> FSNKRVLVEKEGEAGIAVMKFKNPPVNSLSLEFLTEFVISLEKLENDKSIRGVILTSERPGIFSAGL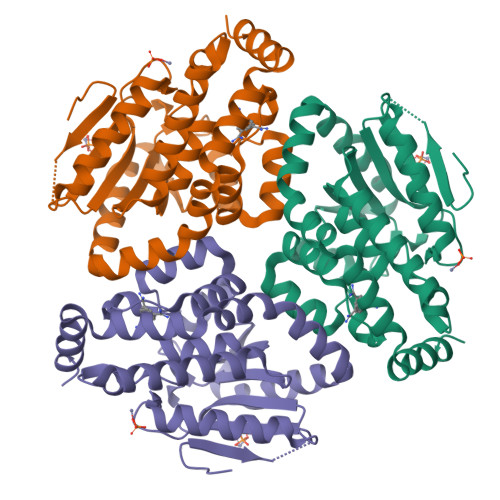DLMEMYGRNPAHYAEYWKAVQELWLRLYLSNLTLISAINGASPAGGCLMALTCDYRIMADNSKYTIGLNESLLGIVAPFWLKDNYVNTIGHRAAERALQLGTLFPPAEALKVGLVDEVVPEDQVHSKARSVMAKWFTIPDHSRQLTKSMMRKATADNLIKQREADIQNFTSFISRDSIQKSLHVYLEKLKQKKG> DLYCYE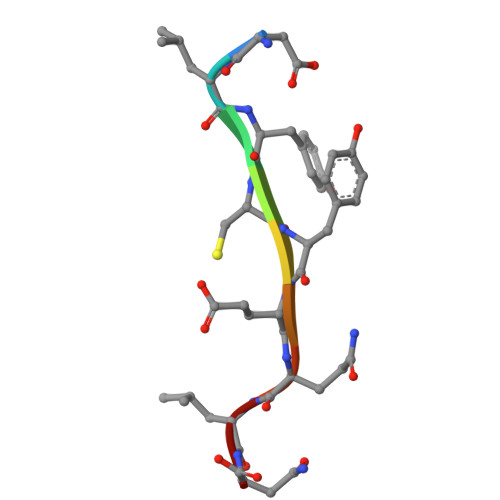QLN> MASM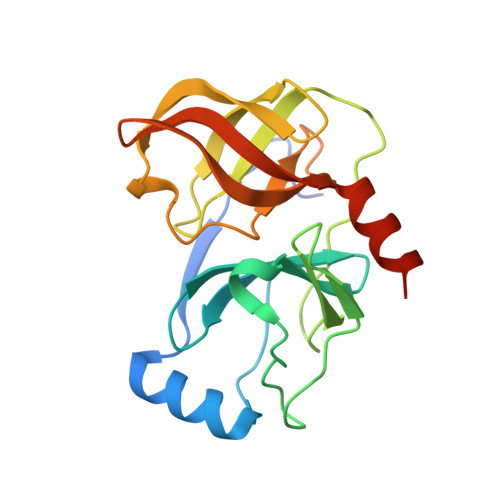TGGQQMGAPITAYAQQTRGLLGCIITSLTGRDKNQVEGEVQIVSTATQTFLATCINGVCWTVYHGAGTRTIASPKGPVIQMYTNVDQDLVGWPAPQGSRSLTPCTCGSSDLYLVTRHADVIPVRRRGDSRGSLLSPRPISYLKGSAGGPLLCPAGHAVGLFRAAVCTRGVAKAVDFIPVENLETTMRSGSHHHHHH>MVALSAEGSSGGSRGGSPKAEAASVPSWPQILGRLTDNRDLARGQAAWAMDQIMTGNARPAQIAAFAVAMTMKAPTADEVGELAGVMLSHAHPLPADTVPDDAVDVVGTGGDGVNTVNLSTMAAIVVAAAGVPVVKHGNRAASSLSGGADTLEALGVRIDLGPDLVARSLAEVGIGFCFAPRFHPSYRHAAAVRREIGVPTVFNLLGPLTNPARPRAGLIGCAFADLAEVMAGVFAARRSSVLVVHGDDGLDELTTTTTSTIWRVAAGSVDKLTFDPAGFGFARAQLDQLAGGDAQANAAAVRAVL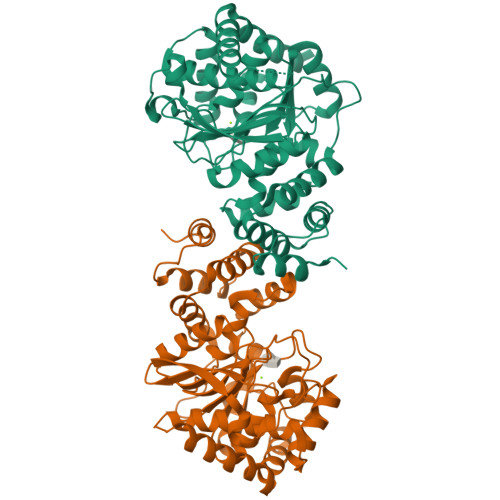GGARGPVRDAVVLNAAGAIVAHAGLSSRAEWLPAWEEGLRRASAAIDTGAAEQLLARWVRFGRQILEHHHHHH[2x]> GGGGALPAKENEGCIVSVNSGKRYCLPVGQRSGYSLPDWIVGQEVYVDSGAKAK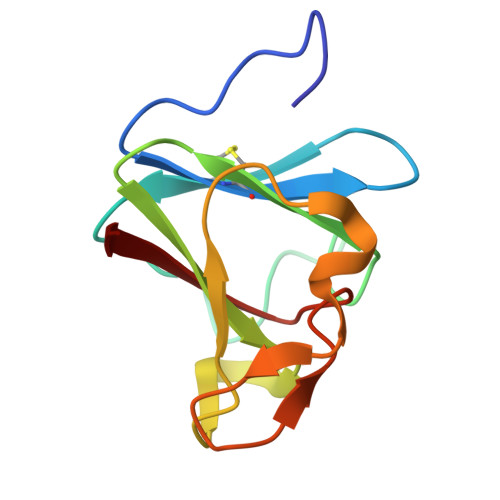VLLSDWDNLSYNRIGEFVGNVNPADMKKVKAWNGQYLDFSKPRSMRVVYK(5Z)-4-hydroxy-3-[(2R)-2-(2-hydroxypropan-2-yl)-2,3-dihydro-1-benzofuran-5-yl]-5-{[(2R)-2-(2-hydroxypropan-2-yl)-2,3-dihydro-1-benzofuran-5-yl]methylidene}furan-2(5H)-one 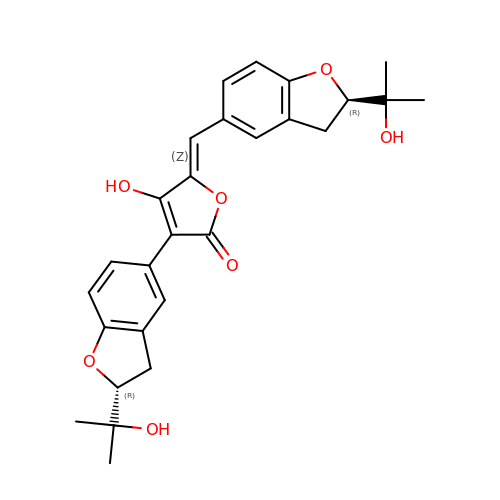| C27 H28 O7 | YPXKKOMPEGAWMY-JQOCIHOLSA-N> MLNPPKHYSVESLRTVGLLPAQLALSRKPRLRPHVGNLKGLVYPLPYYAMWRGNHNKYTYNKSTVCLWGEGDTRSMYHQHYAHAKCPTDYGRGGREFEYLTVKRGKMLQKPLPRVQYVAEGSKPVWLFKSWHTPLSSPSMWEREVQYAE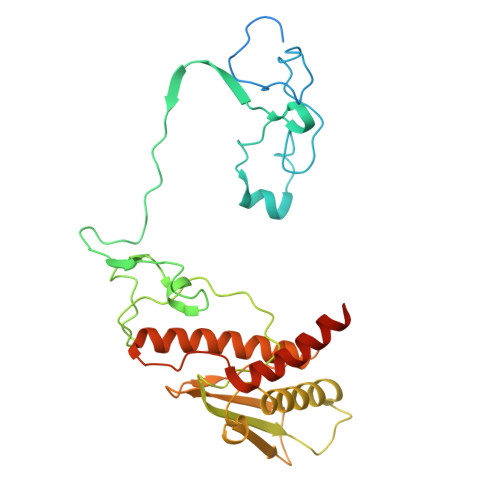HTPEHIGAKRPLAVVAPRTMHRYLFLMHMEKVTITVSPLLFGYGHTIQKAVLDFYRRAISARSPFPKDKVFLFYAIDHITPRIEVTWLDGTSYVPPVLEGASSQDLIQMVMEEAWLAADRMAAEGRVLNPLAIDDYKWDQLVVFKKVRDKEASKGGGRKK1-ethyl-2-[(1-ethylquinolin-2-yl)methyl]quinoline 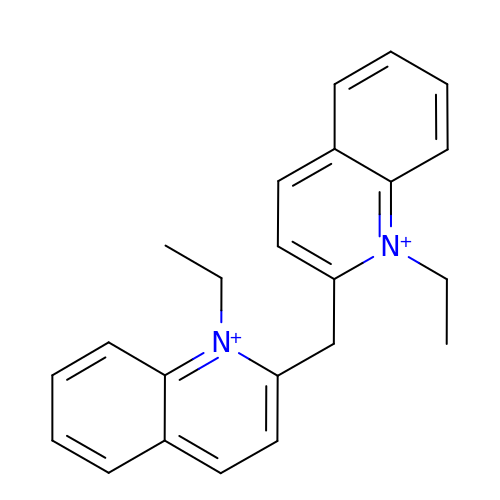| C23 H24 N2 | LVEPVOGKAJXFDF-UHFFFAOYSA-N N-({3-HYDROXY-2-METHYL-5-[(PHOSPHONOOXY)METHYL]PYRIDIN-4-YL}METHYL)-L-CYSTEINE | C11 H17 N2 O7 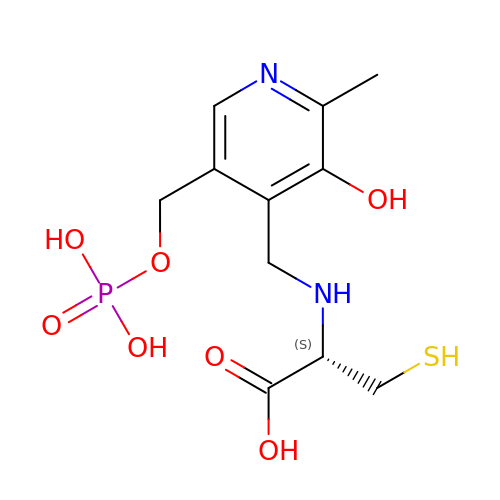P S | FPVGQJHHLSVHOT-VIFPVBQESA-N>MSAIENFDAHTPMMQQYLRLKAQHPEILLFYRMGDFYQLFYDDAKRASQLLDISLTKRGASAGEPIPMAGIPYHAVENYLAKLVNQGESVAICEQIGDPATSKGPVERKVVRIVTPGTISDEALLQERQDNLLAAIWQDSKGFGYATLDISSGRFRLSEPADRETMAAELQRTNPAELLYAEDFAEMSLIEGRRGLRRRPLWEFEIDTARQQLNLQFGTRDLVGFGVENAPRGLCAAGCLLQYAKDTQRTTLPHIRSITMEREQDSIIMDAATRRNLEITQNLAGGAENTLASVLDCTVTPMGSRMLKRWLHMPVRDTRVLLERQQTIGALQDFTAGLQPVLRQVGDLERILARLALRTARPRDLARMRHAFQQLPELRAQLETVDSAPVQALREKMGEFAELRDLLERAIIDTPPVLVRDGGVIASGYNEELDEWRALADGATDYLERLEVRERERTGLDTLKVGFNAVHGYYIQISRGQSHLAPINYMRRQTLKNAERYIIPELKEYEDKVLTSKGKALALEKQLYEELFDLLLPHLEALQQSASALAELDVLVNLAERAYTLNYTCPTFID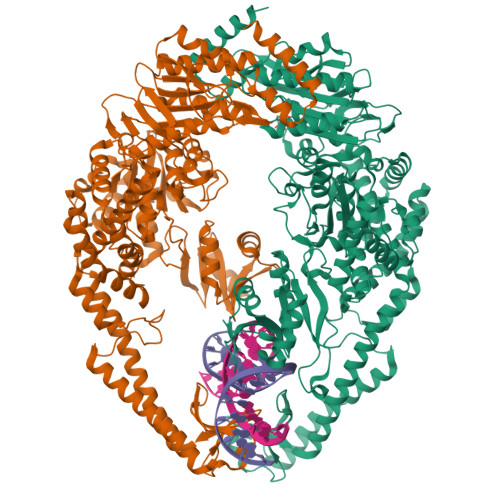KPGIRITEGRHPVVEQVLNEPFIANPLNLSPQRRMLIITGPNMGGKSTYMRQTALIALMAYIGSYVPAQKVEIGPIDRIFTRVGAADDLASGRSTFMVEMTETANILHNATEYSLVLMDEIGRGTSTYDGLSLAWACAENLANKIKALTLFATHYFELTQLPEKMEGVANVHLDALEHGDTIAFMHSVQDGAASKSYGLAVAALAGVPKEVIKRARQKLRELESIS[2x]>[16x]MEINIGIGEQDRAAIAEGLSRLLADTYTLYLKTHNFHWNVTGPMFNTLHLMFEGQYTELAVAVDDIAERIRALGFPAPG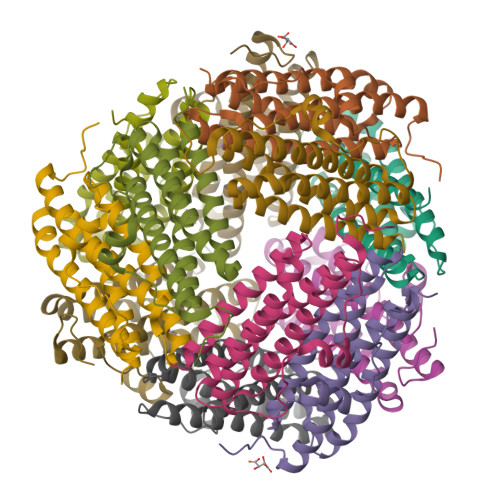TYAAYARLSSIKEEEGVPEAEEMIRQLVQGQEAVVRTARSIFPLLDKVSDEPTADLLTQRMQVHEKTAWMLRSLLAS>MLNNAMSVVILAAGKGTRMYSDLPKVLHTLAGKAMVQHVIDAANELGAAHVHLVYGHGGDLLKQALKDDNLNWVLQAEQLGTGHAMQQAAPFFADDEDILMLYGDVPLISVETLQRLRDAKPQGGIGLLTVKLDDPTGYGRITRENGKVTGIVEHKDATDEQRQIQEINTGILIANGADMKRWLAKLTNNNAQGEYYITDIIALAYQEGREIVAVHPQRLSEVEGVNNRLQLSRLERVYQSEQAEKLLLAGVMLRDPARFDLRGTLTHGRDVEIDTNVIIEGNVTLGHRVKIGTGCVIK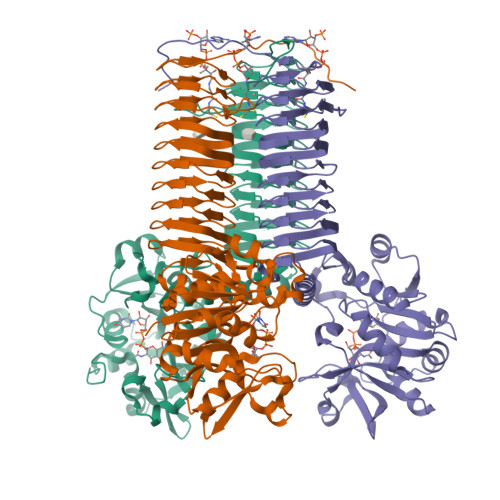NSVIGDDCEISPYTVVEDANLAAACTIGPFARLRPGAELLEGAHVGNFVEMKKARLGKGSKAGHLTYLGDAEIGDNVNIGAGTITCNYDGANKFKTIIGDDVFVGSDTQLVAPVTVGKGATIAAGTTVTRNVGENALAISRVPQTQKEGWRRPVKKK[2x]> MNKLVGLLVSSLFLASILIGIAPAITTTALTPPVSAGGIQAYLLTGSGAPASGLVLFVVNVSNIQVSSSNVTNVISTVVSNIQINAKTENAQTGATTGSVTVRFPTSGYNAYYDSVDKVVFVVVSFLYPYTTTSVNIPLSYLSKYLPGLLTAQPYDETGAQVTSVSSTPFGSLIDTSTGQQILGTNPVLTSYNSYTTQANTNMQEGVVSGTLTSFTLGGQSFSGSTVPVILYAPFIFSNSPYQAGLYNPMQVNGNLGSLSSEAYYHPVIWGRALINTTLIDTYASGSVPFTFQLNYSVPGPLTINMAQLAWIASINNLPTSFTYLSYKFSNGYESFLGIISNSTQLTAGALTINPSGNFTINGKKFYVYLLVVGSTNSTTPVEYVTKLVVEYPSSTNFLPQGVTVTTSSNKYTLPVYEIGGPAGTTITLTGNWYSTPYTVQITVGSTPTLTNYVSQILLKAVAYEGINVSTTQSPYYSTAILSTPPSEISITGSSTITAQGKLTATSASATVNLLTNATLTYENIPLTQYSFNGIIVTPGYAAINGTTAMAYVIGALYNKTSDYVLSFAGSQEPMQVMNNNLTEVTTLAPFGLTLLAPSVPATETGTSPLQLEFFTVPSTSYIALVDFGLWGNLTSVTVSAYDTVNNKLSVNLGYFYGIVIPPSISTAPYNYQNFICPNNYVTVTIYDPDAVLDPYPSGSFTTSSLPLKYGNMNITGAVIFPGSSVYNPSGVFGYSNFNKGAAVTTFTYTAQSGPFSPVALTGNTNYLSQYADNNPTDNYYFIQTVNGMPVLMGGLSIVASPVSASLPSSTSSPGFMYLLPSAAQVPSPLPGMATPNYNLNIYITYKIDGATVGNNMINGLYVASQNTLIYVVPNGSFVGSNIKLTYTTTDYAVLHYFYSTGQYKVFKTVSVPNVTANLYFPSSTTPLYQLSVPLYLSEPYYGSPLPTYIGLGTNGTSLWNSPNYVLFGVSAVQQYLGFIKSISVTLSNGTTVVIPLTTSNMQTLFPQLVGQELQACNGTFQFGISITGLEKLLNLNVQQLNNSILSVTYHDYVTGETLTATTKLVALSTLSLVAKGAGVVEFLLTAYPYTGNITFAPPWFIAENVVKQPFMTYSDLQFAKTNPSAILSLSTVNITVVGLGGKASVYYNSTSGQTVITNIYGQTVATLSGNVLPTLTELAAGNGTFTGSLQFTIVPNNTVVQIPSSLTKTSFAVYTNGSLAIVLNGKAYSLGPAGLFLLPFVTYTGSAIGANATAIITVSDGVGTSTTQVPITAENFTPIRLAPFQVPAQVPLPNAPKLKYEYNGSIVITPQQQVLKIYVTSILPYPQEFQIQAFVYEASQFNVHTGSPTAAPVYFSYSAVRAYPALGIGTSVPNLLVYVQLQGISNLPAGKYVIVLSAVPFAGGPVLSEYPAQLIFTNVTLTQ

Surface layers (S-layers) are resilient two-dimensional protein lattices that encapsulate many bacteria and most archaea. In archaea, S-layers usually form the only structural component of the cell wall and thus act as the final frontier between the cell and its environment. Sulfolobus acidocaldarius is a hyperthermophilic and acidophilic Crenarchaeon and thrives in acidic thermal soils and hot springs worldwide. The Sulfolobales S-layer lattice stands out from others because it is a two-component lattice, consisting of the S-layer-forming SlaA and the membrane anchor SlaB.

A pH shift from acidic (~pH 4) to alkaline (~pH 10) induces the disassembly of the lattice into its component subunits, while a reassembly occurs upon shifting the pH back to acidic. Asking whether this pH shift-induced assembly and disassembly mechanism is based on a conformational change or partial unfolding of SlaA, we investigated the structure of SlaA at different pH conditions. Purified SlaA proteins were frozen at pH 7 and 10 and their structure was determined using the SPA pipeline in Relion (Zivanov et al., 2018) and 3.1 (Figure 3—figure supplements 1 and 2). The resulting cryoEM maps had global resolutions of 3.9 Å for SlaA at pH 7 and 3.2 Å for SlaA at pH 10. As for SlaA at pH 4, domains D5 and D6 were too flexible to be resolved in the cryoEM maps. Strikingly, the cryoEM maps of SlaA30–1069 at the three pH conditions were virtually identical, demonstrating a remarkable pH stability of this protein. (root-mean-square deviation) value of C⍺ atoms between the pH 4 and 10 structures was 0.79 Å (min. = 0.02 Å; max. = 2.6 Å), confirming that SlaA30–1069 maintains its structure unchanged across a surprisingly broad pH range. This suggests that a pH-induced conformational change or unfolding in SlaA30–1069 is not the cause for S-layer disassembly. An analysis of the surface charges of SlaA, including the glycans, at pH 4, 7, and 10 revealed that the overall protein charge changes from positive at pH 4 to negative at pH 10. A comparison of the surface charge between glycosylated and non-glycosylated SlaA showed that the glycans contribute considerably to the negative charge of the protein at higher pH values. This change in electrostatic surface potential may be a key factor in disrupting protein–protein interactions within the S-layer, causing its disassembly at alkaline pH.3-methylthiophene-2-carboxylic acid | C6 H6 O2 S | 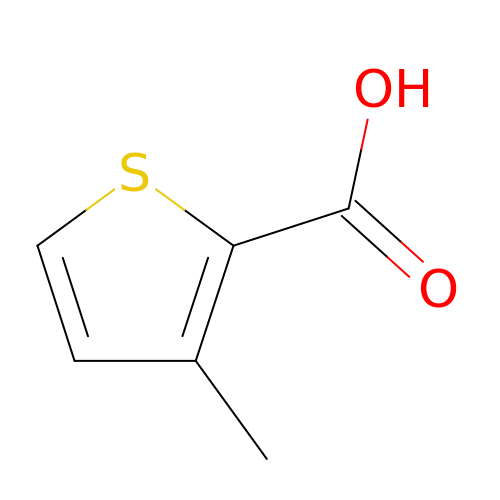IFLKEBSJTZGCJG-UHFFFAOYSA-N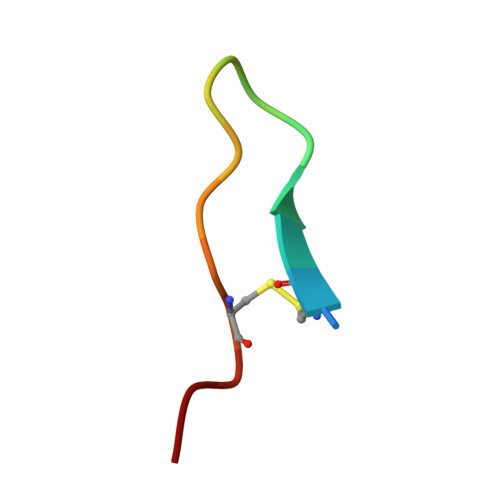> IGCWTKSIPPRPCFVK>MRGSHHHHHHGSMEQSHQNLQSQFFIEHILQILPHRYPMLLVDRITELQANQKIVAYKNITFNEDVFNGHFPNKPIFPGVLIVEGMAQSGGFLAFTSLWGFDPEIAKTKIVAFMTIDKVKFRIPVTP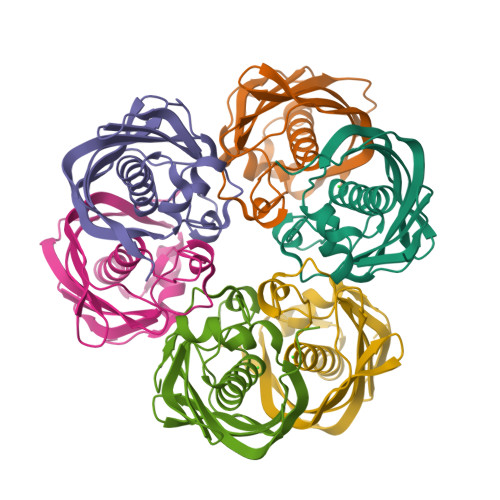GDRLEYHLEVLKHKGMIWQVGGTAQVDGKVVAEAELKAMIAERE[12x]> MRRRAAAVVLSLSAVLATSAATAPAQTPTATATSAKAAAPACPRFDDPVHAAADPRVDVERITPD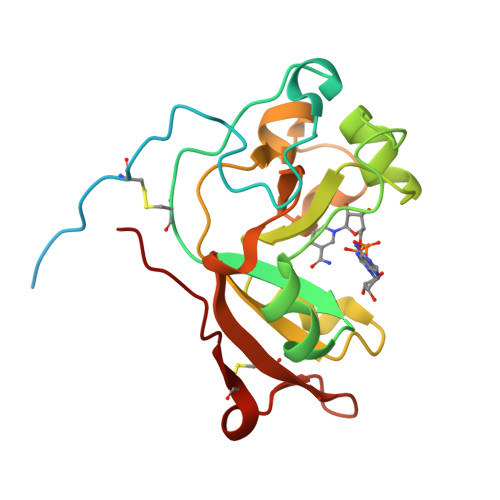PVWRTTCGTLYRSDSRGPAVVFEQGFLPKDVIDGQYDIESYVLVNQPSPYVSTTYDHDLYKTWYKSGYNYYIDAPGGVDVNKTIGDRHKWADQVEVAFPGGIRTEFVIGVCPVDKKTRTEKMSECVGNPHYEPWH> ADTIVAVELDTYPNTDIGDPSYPHIGIDIKSVRSKKTAKWNMQNGKVGTAHIIYNSVDKRLSAVVSYPNADSATVSYDVDLDNVLPEWVRVGLSASTGLYKETNTILSWSF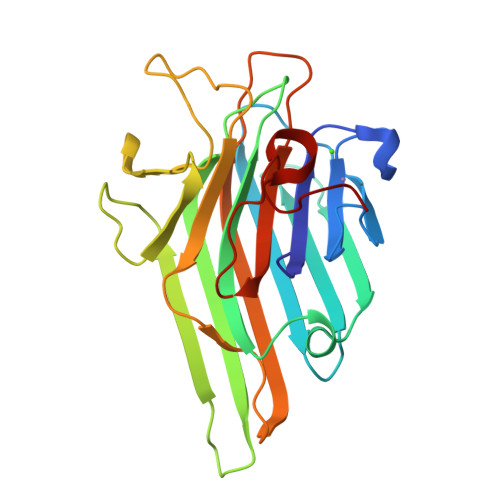TSKLKSNSTHETNALHFMFNQFSKDQKDLILQGDATTGTDGNLELTRVSSNGSPQGSSVGRALFYAPVHIWESSAVVASFEATFTFLIKSPDSHPADGIAFFISNIDSSIPSGSTGRLLGLFPDAN> SSGIHVALVTGGNKGIGLAIVRDLCRLFSGDVVLTARDVTRGQAAVQQLQAEGLSPRFHQLDIDDLQSIRALRDFLRKEYGGLDVLVNNAGIAFKVADPTPFHIQAEVTMKTNFFGTRDVCTELLPLIKPQGRV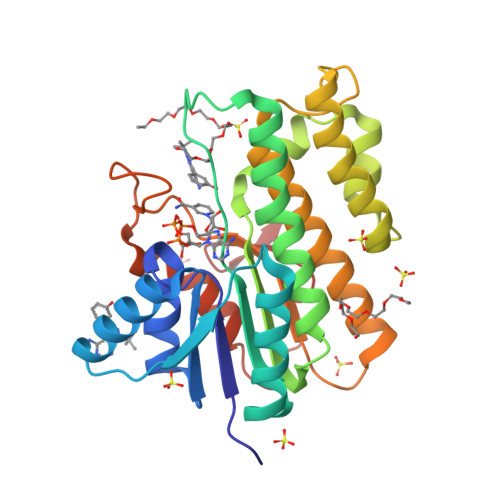VNVSSIMSVRALKSCSPELQQKFRSETITEEELVGLMNKFVEDTKKGVHQKEGWPSSAYGVTKIGVTVLSRIHARKLSEQRKGDKILLNACCPGWVRTDMAGPKATKSPEEGAETPVYLALLPPDAEGPHGQFVSEKRVEQW> GLGQMLESMIDNTVSSTVGAATSRDALPNTEASGPTHSKEIPALTAVETG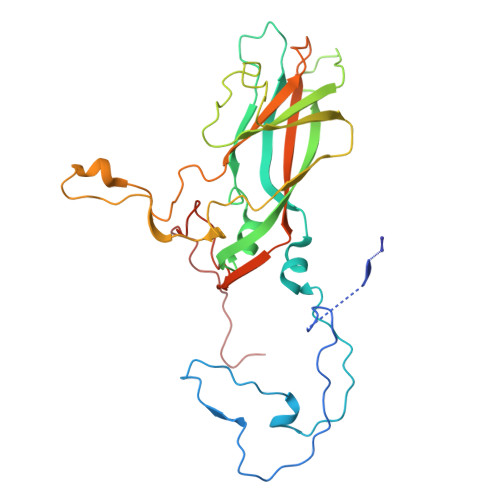ATNPLVPSDTVQTRHVVQHRSRSESSIESFFARGACVTIMTVDNPASTTNKDKLFAVWKITYKDTVQLRRKLEFFTYSRFDMELTFVVTANFTETNNGHALNQVYQIMYVPPGAPVPEKWDDYTWQTSSNPSIFYTYGTAPARISVPYVGISNAYSHFYDGFSKVPLKDQSAALGDSLYGAASLNDFGILAVRVVNDHNPTKVTSKIRVYLKPKHIRVWCPRPPRAVAYYGPGVDYKDGTLTPLSTKDLTTY> GAMGSKGAVVGIDLGTTNSCVAVMEGKQAKVLENAEGARTTPSVVAFTADGERLVGMPAKRQAVTNPNNTFYATKRLIGRRYDDPEVQKDIKNVPFKIVRASNGDAWVEAHGKLYSPSQIGAFVLMKMKETAENYLGHTAKNAVITVPAYFNDSQRQATKDAGQISGLNVLRVINEPTAAALAYGLDKSEDKVIAVYDLGGGTFDISILEIQKGVFEVKSTNGDTFLGGEDFDQALLRHIVKEFKRETGVDLTKDNMALQRVREAAE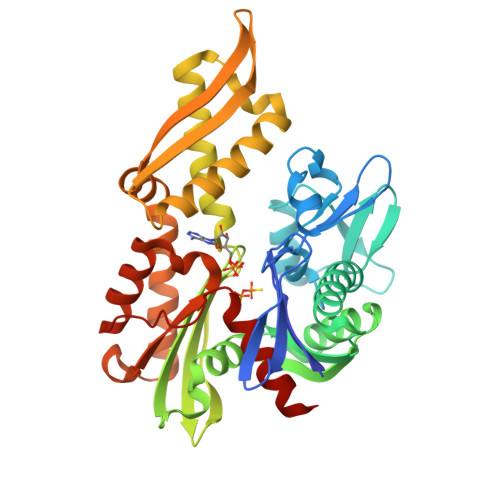KAKCELSSSVQTDINLPYLTMDSSGPKHLNMKLTRAQFEGIVTDLIRRTIAPCQKAMQDAEVSKSDIGEVILVGGMTRMPKVQQTVQDLFGRAPSKAVNPDEAVAIGAAIQGGVLAGD>AYLLFYTEAKVTV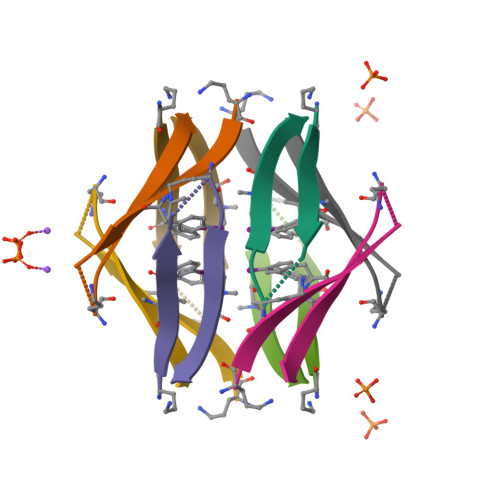TVK[12x]methyl 3-[({2'-(aminomethyl)-5'-[(3-fluoropyridin-4-yl)carbamoyl]biphenyl-3-yl}carbonyl)amino]-4-fluorobenzoate 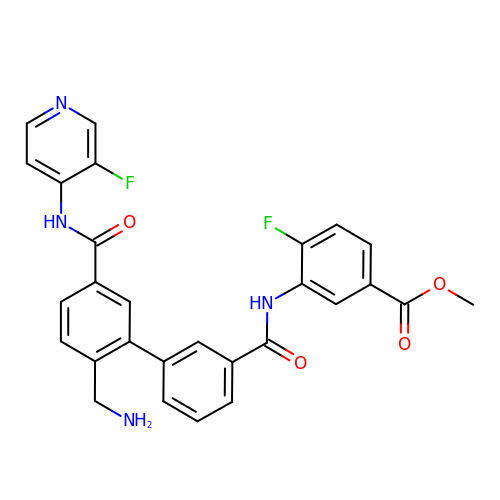| C28 H22 F2 N4 O4 | OZKJLTGMZXEHHT-UHFFFAOYSA-N> MNRLQPVRLVSFVTTDLAGITRGRSLPLATLEEQLASGCGWVPANSSLTPQDLIDESSPWGSHGDLRLLPDPNSRVRVEQGPDAAAPALDYLHGNL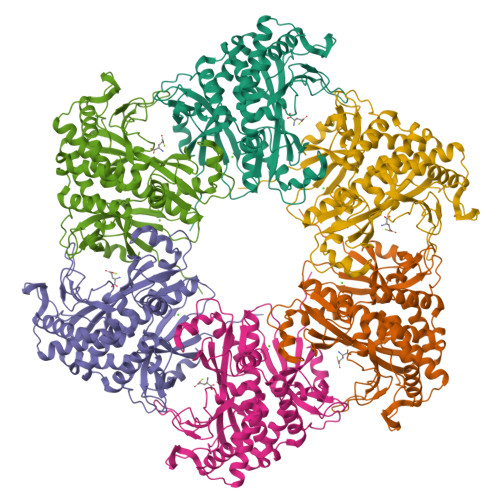VETDGTPWPACPRSLLRAEVERYRDSGLQVIAAFEHEFSLLGLPGERPAAAFSLQAQRAAGQFPGWLVSALAQAGTEPEMFLPEYGQRQYEVTCRPAQGVAAADRAVNVREVTREVARQMGLRTCFAPLPAPGAVTNGVHLHLSLQHADGSPLLYEPGRPNDLSELGEHWAAGVLAHLPALCALTAPTAASYLRLKPHHWSAAYACLGLRNREAALRICPVVSVGGKPLGKQYNLEFRPMDATTCPHLAMAAVLIAGRLGIERRLPLRALADVDPHGLSDEERQARGIQALPATLGDALDCLQRDEALCAELPKPLLDTYLAMKRHELALTAGLSDDDLCRHYAELY>[3x]MARGMNHVYLIGALARDPELRYTGNGMAVFEATVAGEDRVIGNDGRERNLPWYHRVSILGKPAEWQAERNLKGGDAVVVEGTLEYRQWEAPEGGKRSA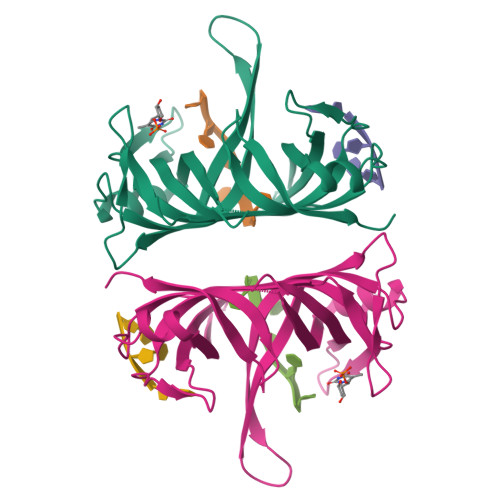VNVKALRMEQLGTQPELIQDAGGGVRMSGAMNEVLVLGNVTRDPEIRYTPAGDAVLSLSIAVNENYQDRQGQRQEKVHYIDATLWRDLAENMKELRKGDPVMIMGRLVNEGWTDKDGNKRNSTRVEATRVEALARGAGNANSGYAAATPAAPRTQTASSAARPTSGGYQSQPSRAANTGSRSGGLDIDQGLDDFPPEEDDLPF3-[[(1~{S},3~{S})-3-methylcyclohexyl]methyl]-6,8-bis(oxidanyl)isochromen-1-one | C17 H20 O4 | 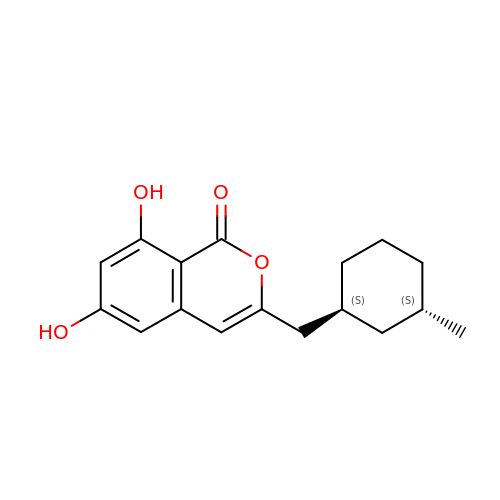JSPLICPLSKXJBM-QWRGUYRKSA-N> MGIVEEAHNVKVLGTGSRFIVLAHGFGTDQSVWKHLVPHLLEEFRVILYDNMGAGTTNPDYFDFERYSTLEGYAYDLLAILQELRVDSCIFVGHSVSAMIGTVASISRPDLFAKIIMISASPRYLNDSNYFGGFEQEDLDQLFNAMASNYKAWCSGFAPMAIGGDMESVAVQEFSRTLFNMRPDIALSVLQTIFKSDMRQILCLVSVPCHIIQSMKDLAVPVVVAEYLHQHVGTESIVEVMSTEGHLPQLSSPDVVIPVILKHIRYDIVA

KAI2 proteins are plant α/β hydrolase receptors which perceive smoke-derived butenolide signals and endogenous, yet unidentified KAI2-ligands (KLs). Prior to their diversification, KAI2 underwent duplication resulting in KAI2A and KAI2B. Here we demonstrate that Pisum sativum KAI2A and KAI2B are active receptors and enzymes with divergent ligand stereoselectivity. To further address this point, we determined the structure of an evolutionarily diverged PsKAI2B in apo and a unique butenolide-bound state at high resolution (1.6 Å and 2.0 Å, respectively).

To elucidate the structural basis for the differential ligand selectivity between KAI2A and KAI2B, we determined the crystal structure of PsKAI2B at 1.6 Å resolution. The PsKAI2B structure shares the canonical α/β hydrolase fold and comprises base and lid domains. The core domain contains seven-stranded mixed β-sheets (β1–β7), five α-helices (αA, αB, αC, αE and αF) and five 310 helices (ŋ1, ŋ2, ŋ3, ŋ4, and ŋ5). The helical lid domain (residues 124–195) is positioned between strands β6 and β7 and forms two parallel layers of V-shaped helices (αD1-4) that create a deep pocket area adjoining the conserved catalytic Ser-His-Asp triad site. Nonetheless, further structural comparative analyses have identified two residue alterations in positions 129 and 147 within the lid domain which appear to slightly alter the backbone atoms and generally distinguish legume KAI2 proteins from KAI2s in other species. PsKAI2B exhibits a structural arrangement that results in a larger volume of the hydrophobic pocket (125.4 A3) yet with a smaller entrance circumference (30.3 Å) than PsKAI2A (114.8 A3 and 33.6 Å, respectively). Further in silico docking experiments of (–)-GR24 with PsKAI2B resulted in a successful docking of the ligand that is completely buried in the pocket and positioned in a pre-hydrolysis orientation nearby the catalytic triad. Among these residues, L160/S190/M218 in PsKAI2A and the corresponding residues, M160/L190/L218 in PsKAI2B are of particular interest because of their functional implications in the pocket volume and solvent accessibility. Residue 160 is positioned at the entrance of the ligand-binding pocket in helix αD2, thus the substitution of leucine (L160 in KAI2A) to methionine (M160 in KAI2B) results in modifying the circumference of PsKAI2B pocket entrance. Residue 190 (S190 in PsKAI2A and L190 in PsKAI2B) is positioned in helix αD4 and represents a major structural arrangement at the back of the ligand envelope.>[2x]MSIVNILSVNVLNNPAKFSDPYKFEITFECLEPLKSDLEWKLTYV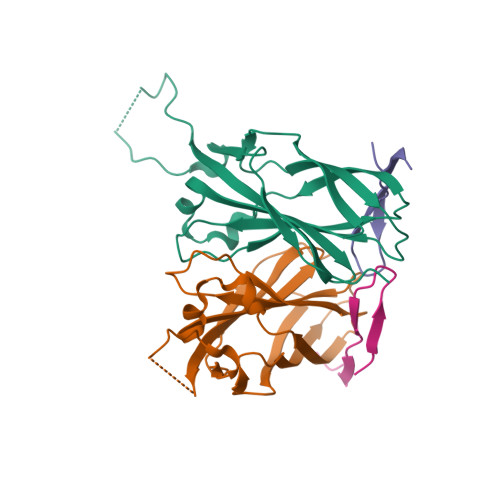GSATSQSYDQILDTLLVGPIPIGINKFVFEADPPNIDLLPQLSDVLGVTVILLSCAYEDNEFVRVGYYVNNEMEGLNLQEMDDAEIKKVKVDISKVWRSILAEKPRVTRFNIQWDN;>IPTKFVQKVTITKEGKKRVAPQLLTTLSA[2x]N-[2-(hydroxymethyl)-3-{5-[(5-methyl-4,5,6,7-tetrahydropyrazolo[1,5-a]pyrazin-2-yl)amino]-6-oxo-1,6-dihydropyridazin-3-yl}phenyl]-1-benzothiophene-2-carboxamide | C27 H25 N7 O3 S | 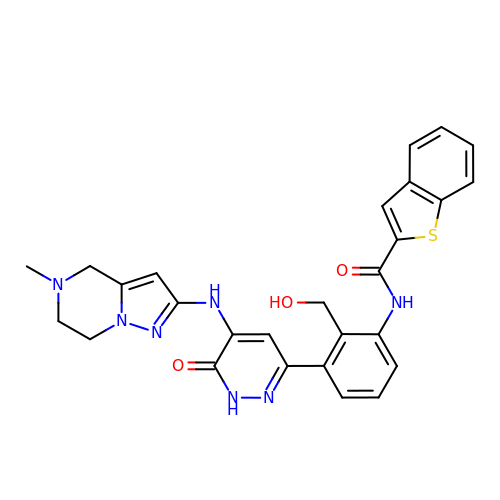OVVJBKJSJVGGOF-UHFFFAOYSA-N> MYSVQIAVSDGTLTRIALSIEYFEKDDITLYRNLELTPLVLGTDWQWDGDTHINLLTGIPVPVGSYITVRRNTDIDRAFNIYDGGAAFNRETLDENFKQMIYLAQEFTEGNGLTGLYFPLDMHGFQIKNLGEPTDPGDAVTKQYVDTANTAQNANFNASQQAQDQAVAASQAVQDNRLASLENTFVQATSSYPWYTVSTSTTDTFTPGFNFTKAAVYINGVCQTPDYSYIVVAN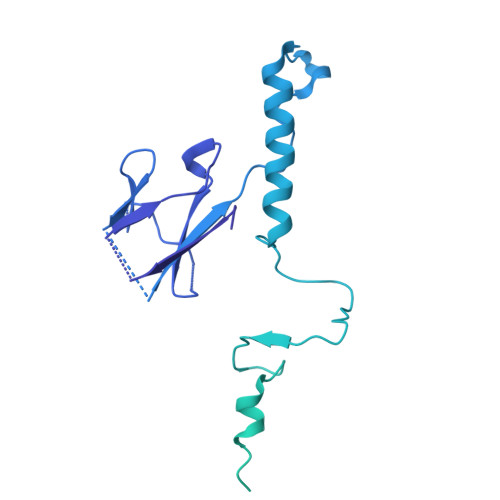QILLADPVPLGTMVFARLGEDIQNDDDFATTAQLSAVQANLQDEIDVTNTEVSNKASKGANSDISSLSGLTTPLSAAQGGTGNNTGNAATATVLATPRTIQTNLASTSAASFNGSANITPGVTGNLPVTNGGTGAGSAPSARANLGAAMNGINNDISNLAALTGGITGLTTGTAAASGIVGEVASAASSSATNLVSGSVINIISLSLPAGDWELESAFQIINTGNVTALAFGVSTTTGVLPTPWYDVYSITTTIGSGTSNRQGMARRVLLSTTTTVYLVAQATFTGTATANGYVRARRVR>[2x]GGKKDKEKIIDDFKVAVVTQPLSENKVQYNMVEEMAKEYEEENKIDKDKDGQTKVKQTIKHVVLPENFTSNIDSAINKIVKLADDKEVQ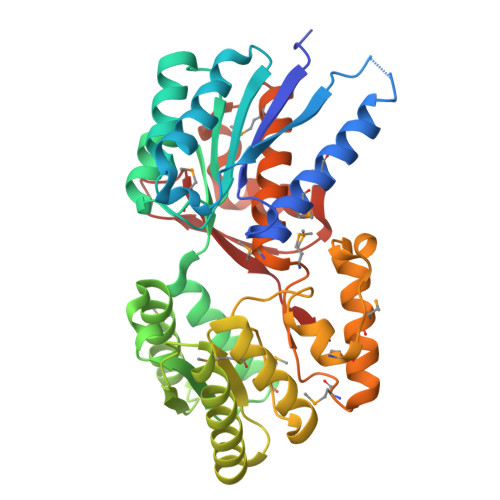AIVVSTDQAGLLPALQKVKEKRPEIITISAPMGDDKNQLSQFVDVNLGVSAEERGKVLAERSKEMGAKAFIHYASTDDLKDVNIAKRLEMIKETCKNIGLPFVQVNTPNINTEEDKNKVKQFLNEDIEKQVKKYGKDINVFGVNEYMDEVILTKALELKYIVAEQSNPSPIQTYPSVMGLKISEKDAQNYDKINDMISEKAKAFGMSNRLGGYPMPMDAFLPSLAIYLATEMVKQDLTQEDVCDPDYLEAFTELRFGIGSEFTPLTEVLYNYQSVILSQLIY[(3~{S},4~{R},5~{R})-5-(6-aminopurin-9-yl)-4-oxidanyl-oxolan-3-yl] [oxidanyl(phosphonooxy)phosphoryl] hydrogen 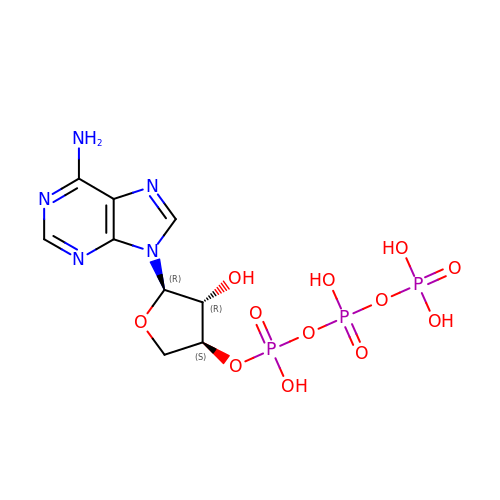phosphate | C9 H14 N5 O12 P3 | AWDFERYZHFHVNT-AFEQZKEHSA-N> UCCGAAGUGCAACGGG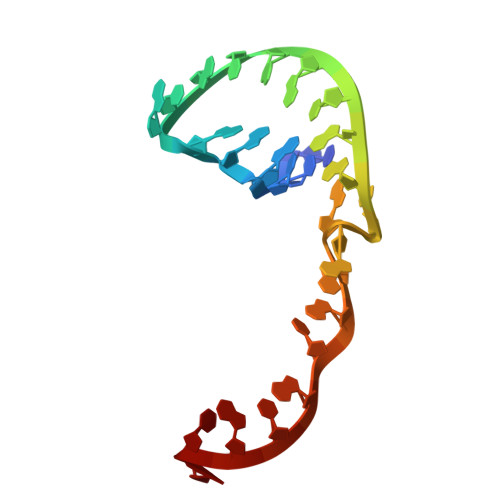AAAAUGCACU> MIVDGDLHIHSHYSKAVSKLMTFPIIAENAKLKGLNLVGTG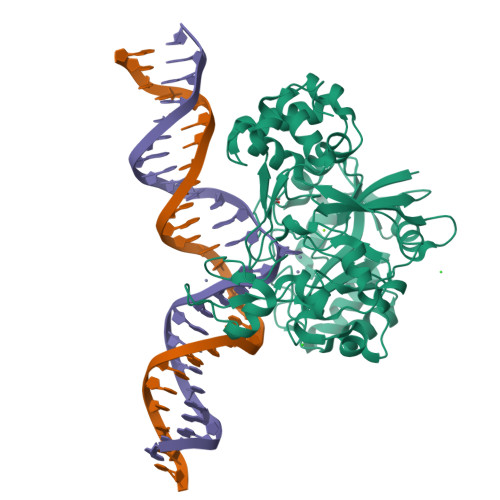DSLNPHWEKELLKHSKPIDDGTFEVNGVKFILTCEVEDKRRVHHLLIFPTLSQVREFREKVKIYSTNIESEGRPNLNLTAEEIAEMANELDILIGPAHAFTPWTSLYKEYDSLKDAYGDAKIDFLELGLSADSDMADMIKAHHSIPYLSNSNAHSPNPHRLGREFNRFEVKDVTFEEIRKAIKGVGGRKIMLNAGLDPRLGKYHLTACSRCYTKYTLQDAVSLSWKCPKCGGIIKKGVRDRILELADTSEKPKDRPPYVRLAPLAEIIAMVLGKGIESKAVKLLWNRFLREFGSEIRVLIDLPIESIASVHEGVAKAIWAYRNNKLIIVPGGGGKYGEIRIPEEILKAKIEDLN> 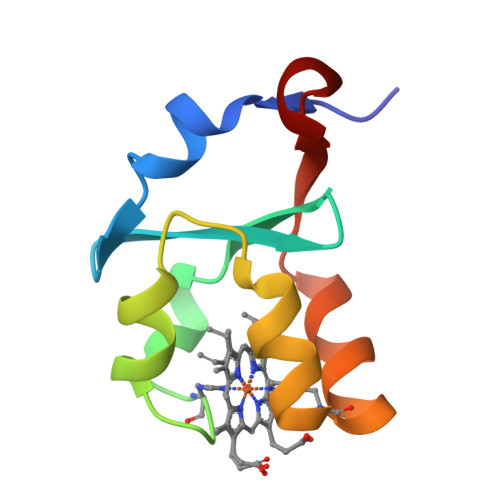AVKYYTLEEIQKHNNAKSTWMIIHYKVYDITRFLSEHPGGEEVLLEQAGADATESFEDVGHSPDAREMLKTFIIGELHPDDR>MAAATGPSFWLGNETLKVPLALFALNRQRLCERLRKNPAVQAGSIVVLQGGEETQRYCTDTGVLFRQESFFHWAFGVTEPGCYGVIDVDTGKSTLFVPRLPASHATWMGKIHSKEHFKEKYAVDDVQYVDEIASVLTSQKPSVLLTLRGVNTDSGSVCREASFDGISKFEVNNTILHPEIVECQVFKTDMELEVLRYTNKISSEAHREVMKAVKVGMKEYELESLFEHYCYSRGGMRHSSYTCICGSGENSAVLHYGHAGAPNDRTIQNGDMCLFDMGGEYYCFASDITCSFPANGKFTADQKAVYEAVLRSSRAVMGAMKPGVWWPDMHRLADRIHLEELAHMGILSGSVDAMVQAHLGAVFMPHGLGHFLGIDVHDVGGYPEGVERIDEPGLRSLRTARHLQPGMVLTVEP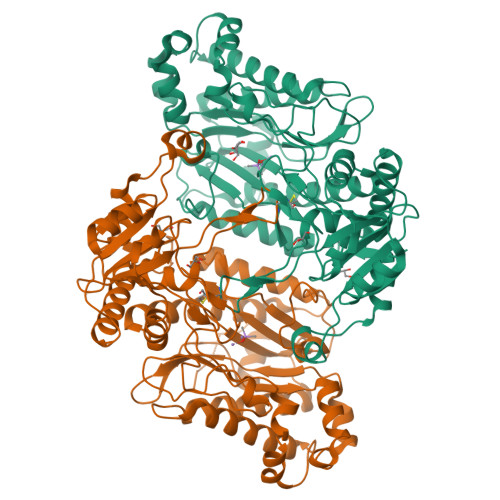GIYFIDHLLDEALADPARASFLNREVLQRFRGFGGVRIEEDVVVTDSGIELLTCVPRTVEEIEACMAGCDKFTPFSGPK[2x]Here we address these limitations by introducing an artificial metathase—an artificial metalloenzyme designed for ring-closing metathesis—for whole-cell biocatalysis. Our approach integrates a tailored metal cofactor into a hyper-stable, de novo-designed protein. By combining computational design with genetic optimization, a binding affinity (KD ≤ 0.2 μM) between the protein scaffold and cofactor is achieved through supramolecular anchoring. From the catalyst perspective, we sought to address this challenge by designing a derivative of the Hoveyda–Grubbs catalyst (hereafter Ru1) that contains a polar motif, aimed at interacting via H-bonds with the protein, as well as improving the cofactor solubility in aqueous media.

To further improve the affinity and ensure near quantitative binding at low micromolar concentrations of dnTRP_18, we set out to increase the hydrophobicity around the Ru1 binding site. For this purpose, positions F43 and F116 were individually mutated to tryptophan. Both dnTRP_18_F43W and dnTRP_18_F116W (hereafter dnTRP_R0) displayed a nearly tenfold higher affinity with KD = 0.26 ± 0.05 and 0.16 ± 0.04 μM at pH 4.2, respectively. A comparison of apo and Ru1·dnTRP_R0-ΔHis X-ray structures with computational models reveals an overall agreement with the toroidal shape but notable deviations with regards to the shape of the inner cavity, as well as the position the Ru1 cofactor. The Cα root mean square deviation values between the AF2 predicted models and the X-ray structures range from 1.59 to 1.63 Å.

> GGGSGVSLEQALLILSVAALLGTTVEEAVKRALWLKTKLGVSLEQAAFILSVAAYLGTTVEEAVKRALKLKTKLGVSLEQALLILFAAAALGTTVEEAVKRALKLKTKLGVSLEQALLILWTAAELGTTVEEAVKRALKLKTKLGVSLEQAQAILVVAAELGTTVEEAVYRALKLKTKLGVSLEQALLILEVAAKLGTTVEEAVKRALKLKTKLG>[2x]GHMPRPSLRRGEETSGARSLHEIAPPAE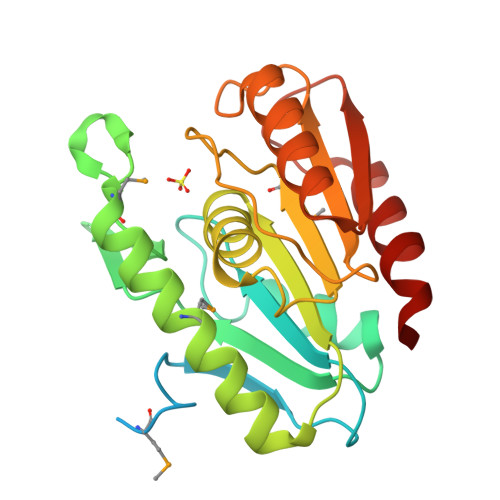KAVRKPLNLLPFRKDTPMTKDSYFHKSRAGVAGAPLFVLLHGTGGDENQFFDFGARLLPQATILSPVGDVSEHGAARFFRRTGEGVYDMVDLERATGKMADFIKANREHYQAGPVIGLGFSNGANILANVLIEQPELFDAAVLMHPLIPFEPKISPAKPTRRVLITAGERDPICPVQLTKALEESLKAQGGTVETVWHPGGHEIRSGEIDAVRGFLAAYGGGS> SGPRPRLWEGQDVLARWTDGLLYLGTIKKVDSAREVCLVQFEDDSQFLVLWKDISPAALPGEELLCCVCRSETVVPGNRLVSCEKCRHAYHQDCHVPRAPAPGEGEGASWVCRQCVFAIATKRGGALKKGPYARAMLGMKLSLPYGLKGLDWDAGHLSNR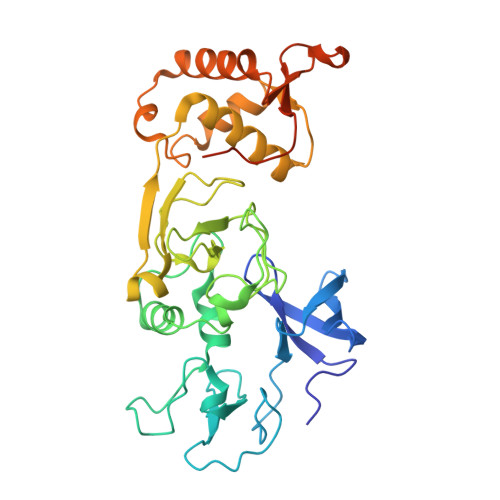QQSYCYCGGPGEWNLKMLQCRSCLQWFHEACTQCLSKPLLYGDRFYEFECCVCRGGPEKVRRLQLRWVDVAHLVLYHLSVCCKKKYFDFDREILPFTSENWDSLLLGELSDTPKGERSSQLLSALNSHKDRFISGREIKKRKCLFGLHARTPPPVELLTGDGAPTSFPSGQGPGGG>LDCTVIDGNLKQIDAGSGSVVGVNNLNETFVLIDNVFTKISGSLKHFSVGPAGQLGVNTANNIFKYQSGGFVQLAGLLKQVDAGGDQIIAGVNMYDDIYCLNMDANNKWPSSNTPWVQLNGKLKYYSCGPYSCWGVNSNDQIFIMKDVSSNVCSGSGSFINIPGLLSMIEVATDGSVFGVNSQGNLYQRTG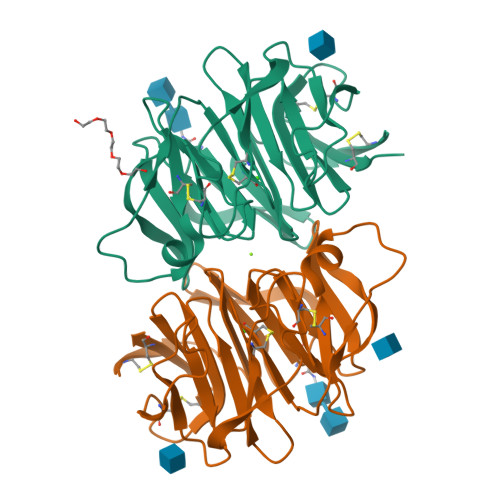VTRSKPDGTDWISMVACPNGHKHVSFDLGVLWLVCVDGSIRKCILTD[6x]> GPGS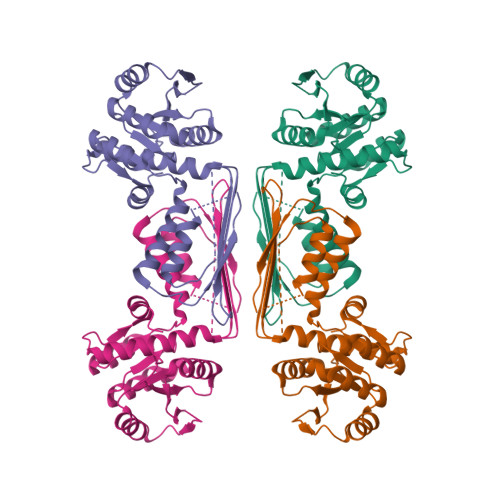MTAMADSGEEAVKSVLPGNGISIMVNGCSGKMGKAVIKAADSAGVNIVPISFGSAGEDGQRVEVCGKEITVHGPTEREKVLSSVFEKHPELIVVDYTIPSAVNDNAELYSKVGVPFVMGTTGGDRNKLYETVEEAKIYAVISPQMGKQVVAFLAAMEIMAEQFPGAFSGYSLDVMESHQASKLDASGTAKAVISCFQELGVSYDMDQIQLIRDPKQQVEMVGVPEEHISGHAFHLYHLTSPDETVSFEFQHNVCGRSIYAEGTVDAVLFLAKKIRLKADQRIYNMIDVLREGNMR> SKTITIYLDPASLPTLNQLMHFTKESEDKETARIFGFSRFKLPEKITEQYNNIHFVEIKNNRPTEDIFTILDQYPEKLELDLHLNIAHSIQLFHPILQYRFKHPDRISIKSLNLYDDGTMEYVDLEKEENKDIKSAIKKAEKQLSDYLLTGKINFDNPTLARYVWQSQYPVKYHFLSTEYFEKAEFLQPLKTYLAGKYQKMDWSAYEKLSPEQQTFYLKLVGFSDETKQLFHTEQTKFIFTGTTTWEGNTDIREYYAKQQLNLLKHFTHSEGDLFIGDQYKIYF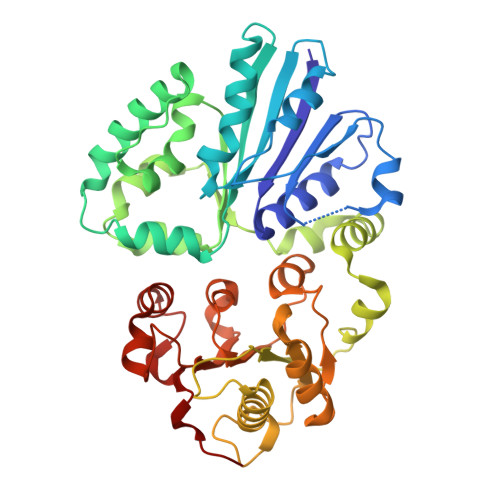KGHPRGGDINDYILKHAKDITNIPANISFEILMMTGLLPDKVGGVASSLYFSLPKEKISHIIFTSNKKIKNKEDALNDPYVRVMLRLGMIDKSQIIFWDSLKQL> MGSSHHHHHHSQSPMFDIKRKTIEWGGKTLVLETGRIARQADGAVLATMGETVVLATAVFAKSQKPGQDFFPLTVNYQEKTFAAGKIPGGFFKREGRPSEKETLVSRLIDRPIRPLFVKGFKNEVQVVVTVLQHDLENDPDILGMVAASAALCLSGAPFMGPIGAARVGWVDGAYVLNPTLDEMKESKMDLVVAGTADAVMMVESEIQELSEEIVLGGVNFAHQQMQAVIDAIIDLAEHAAKEPFAFEPEDTDAIKAKMKDLVGADIAAAYKIQKKQDRYEAVGAAKKKAIAALGLSDENPTGYDPLKLGAIFKELEADVVRRGILDTGLRIDGRDVKTVRPILGEVGILPRTHGSALFTRGETQAIVVATLGTGDDEQFIDALEGTYKESFLLHYNFPPYSVGETGRMGSPGRREIGHGKLAWRALRPMLPTKEDFPYTIRLVSEITESNGSSSMATVCGSSLAMMDAGVPLVRPVSGIA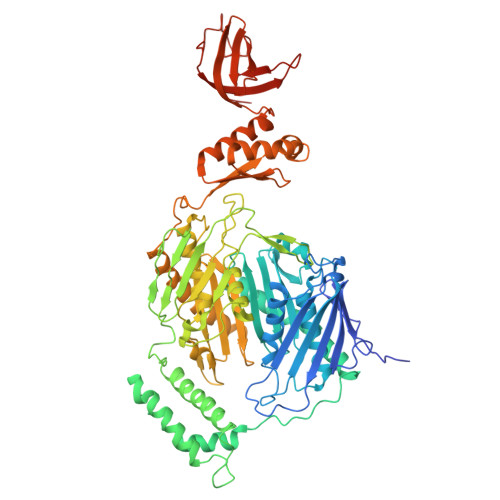MGLILEQDGFAVLSDILGDEDHLGDMDFKVAGTSEGLTSLQMDIKIAGITPAIMEQALAQAKEGRAHILGEMNKAMDAPRADVGDFAPKIETINIPTDKIREVIGSGGKVIREIVATTGAKVDINDDGVVKVSASDGAKIKAAIDWIKSITDEAEIGKIYDGKVVKVVDFGAFVNFFGAKDGLVHVSQISNERVAKPSDVLKEGQMVKVKLLGFDDRGKTKLSMKVVDQETGEDLSKKEAAAEEA> KAQKKNRNKLRRQHSYDTFVD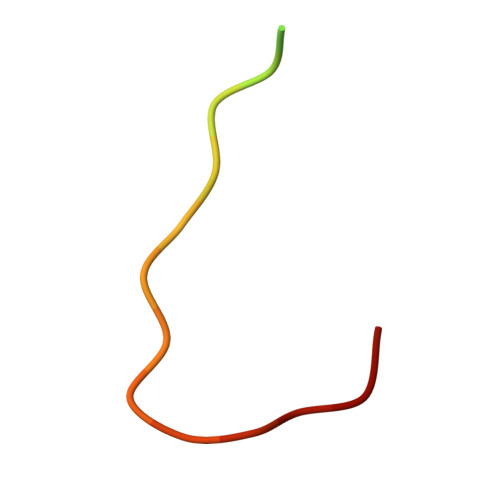L>MTSAEMTSPNNNSEHQAIAKMRTMIEGFDDISHGGLPIGRSTLVSGTSGTGKTLFSIQFLYNGIIEFDEPGVFVTFEETPQDIIKNARSFGWDLAKLVDEGKLFILDASPDPEGQEVVGGFDLSALIERINYAIQ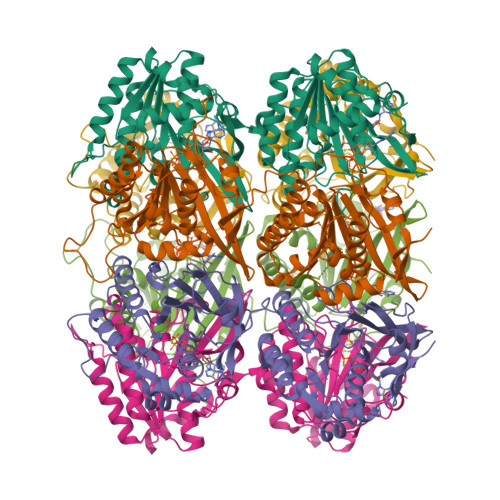KYRARRVSIDSVTSVFQQYDASSVVRRELFRLVARLKQIGATTVMTTERIEEYGPIARYGVEEFVSDNVVILRNVLEGERRRRTLEILKLRGTSHMKGEYPFTITDHGINIFPLGAMRLTQRSSNVRVSSGVVRLDEMCGGGFFKDSIILATGATGTGKTLLVSRFVENACANKERAILFAYEESRAQLLRNAYSWGMDFEEMERQNLLKIVCAYPESAGLEDHLQIIKSEINDFKPARIAIDSLSALARGVSNNAFRQFVIGVTGYAKQEEITGLFTNTSDQFMGAHSITDSHIEAITDTIILLQYVEIRGEMSRAINVFKMRGSWHDKAIREFMISDKGPDIKDSFRNFERIISGSPTRITVDEKSELSRIVRGVQEKGPES[6x]>GAMGGWAIAVHGGAGVDPTLPLERQEEAKQLLTRCLNLGISALNSNVPAIDVVELVVRELETDPLFNSGRGSALTEKGTVEMEASIMDGPKRRCGAVSGLTTVKNPISLARLVMDKSPHSYIAFSGAEDFARQQGVEVVDNEYFVTPDNVGMLKLAKEANTILFDYRIPSSAYETCGSGVESPLQMNGLPISVYAPE[2x];>TVGCVVVDREGRCAAATSTGGLMNKMTGRIGDSPLIGAGTYACDVCGVSCTG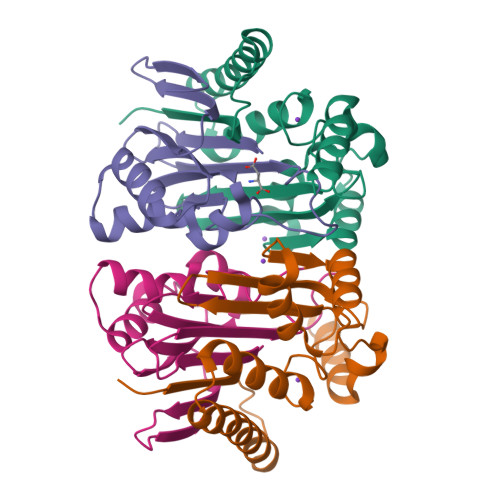EGEAIIRGTLAREVAAVMEYKGLKLHQAVDFVIKHRLDEGKAGLIAVSNTGEVACGFNCNGMFRACATEDGFMEVAIWD[2x]>PVIEINDQEQFTYLTTTAAGDKLIVLYFHTSWAEPCKALKQVFEAISNEPSNSNVSFLSIDADENSEISELFEISAVPYFIII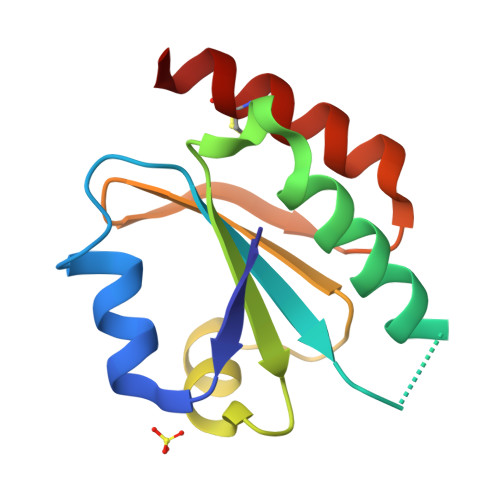HKGTILKELSGADPKEYVSLLEDCKNSVN[2x]> MHHHHHHENLYFQSTSTQFYYKLSQELNGDMERVADSLVTLQDQLNSLAAVVLQNRRALDLLTAERGGTCL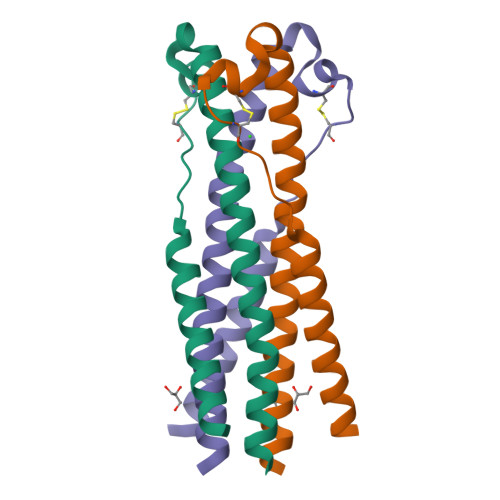FLGEECCYYVNQSGIVTEKVKEIRDRIQRRAEELRNT> MPYTWKFLGISKQLSLENGIAKLNQLLNLEVDLDIQTIRVPSDPDGGTAADEYIRYEMRLDISNLDEGTYSKFIFLGNSKMEVPMFLCYCGTDNRNEVVLQWLKAEYGVIMWPIKFEQKTMIKLADASIVHVTKENIEQITWFSSKLYFEPETQDKNLRQFSIEIPRESCEGLALGYGNTMHPYNDAIVPYIYNETGMAVERLPLTSVILAGHTKIMRESIVTSTRSLRNRVLAVVLQSIQFTSE;> MSNELRLEDNYVPTSDTLVVFKQLMKLPVTVLYDLTLSWFAKFGGSFDGDIYLLTETLDLLIEKGVRRNVIVNRILYVYWPDGLNVFQLAEIDCHLMISKPEKFKWLPSKALRGDGKPYVVKLQPAKFIENLQTDLAKIYHCHVYMFKHPSLPVLITRIQLFDSNNLFLSTPNIGSINKESLYNKLDKFQGKPLISRRPYYVAFPLNSPIIFHSVDKDIYARLVLQSISRTISERETIIFKPVQKIPVKSIHNIMTLLGPSRFAESMGPWECYASANFERSPLHDYKKHQGLTGKKVMVREFDDSFLNDDENFYGKEEPEIRRLRLEKNMIKFKGSANGVMDQKYNDLKEFNEHVHNIRNGKKNEDSGEPVYISRYSSLVPIEKVGFTLKNEINSRIITIKLKFNGNDIFGGLHELCDKNLINIDKVPGWLAGENGSFSGTIMNGDFQREQVAKGGLLENLYFQ;> MSRIDDLQQDIESLLSEINSLEESREKLKAKIKDKRKNEESANPIVQEFEDLFDQFPQLNNFLFNEHPELEETDDKDISRAQADIPATPIPYEPKKRAKLENEEILPEQEWVLKTQPMVQHQMFDPGVADLLDTDILTSPSKRKRKLKIDDISTSDRSELEDYIVLENVYRMFGITFFPLVDPIDLKIKDASGEIFVDREMLGIRLEVFSERTSQFEKPHYVLLKKRIKSNSWFLFKHTIPSFIDVQGIFDDTNGGLVISHDDAYLFAKRVFLQLVEVQKRRQIFKDLEAKKIIHDLDLDLESSMVSFFVKDIKVELFVKQNEIVSCSILDDIHDFSQNNKSKWEIALLGSLDDLELKLNHSFATIFK;> MDFTSDTTNSHDTSNSHLSLEDAVGTHHAGEADVNIDGDEKQQLSLLDDDQVRALKLQEEKDALLTRRNTLLQEIQTYQNILMKENNSKTKNGDILQNDITQDFLNLISISSSNPNSAISDRKRVERINGLTNLQKELVTKYDTLPLLNMNLRLSYLRDHTYPHLQVSVQSRDRVHNDGIEVLVVNYKFCRNTMNPFEIQFKMFYKFEDSTLLKWEILRISTNVRLKAKQLLATRNFQKCLLSLYEFDKIKSKKTGIFQNLINLLKRKTRCYLMNNSDSLIVERVIREGRLTTIKLQINFIITMPGERGKPRNCFLPMSKISIALWKGGERF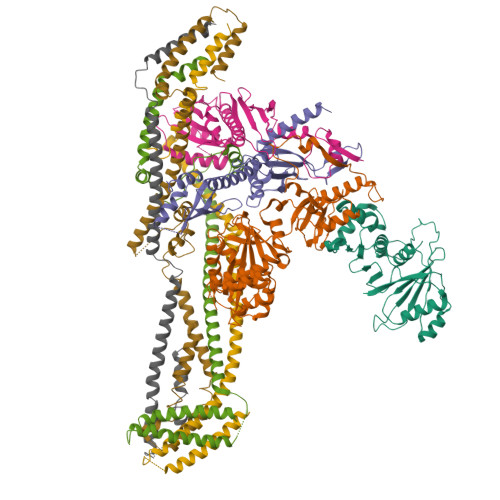NQIDLDEICYGLIKEYGVKTGLKEICNVCLFPDMYAR;> MAADRDNFLQNIENDSINNGQAMDLSPNRSSSESDSSILMNVNDIKTLRLDVAPEAKSTQSKKSLFYENSDDAEEGEIEERTNKEEGQYHHKGSKQLRFEVGKESTGKLQSHLSDGSATSGEGNVRPWEFRKVIQAEYRERLPRNYELKHWKKPSKIMIGSILRLLETNTVSALDSVFEKYEKEMNQMTHGDNNEVKRIYSKKERLLEIILTKIKKKLRQAKFPSRISERDLDIEYIYSKRQFIQNRYSQELQNNERLEAILSREQNLLEETRKLCMNLKTNNKKRLTEKLIQKDLHPVLNKAMEYTYGLESTNGFMHPDGPVTFRNDSHELNLMLNDPIKSTADVRLDKEEVLSLLPSLKEYTKKSKELKETMGQMISDSHEEEIKEVFVPHHESHQDKTEEDIH;> MDRDTKLAFRLRGSHSRRTDDIDDDVIVFKTPNAVYREENSPIQSPVQPILSSPKLANSFEFPITTNNVNAQDRHEHGYQPLDAEDYPMIDSENKSLISESPQNVRNDEDLTTRYNFDDIPIRQLSSSITSVTTIDVLSSLFINLFENDLIPQALKDFNKSDDDQFRKLLYKLDLRLFQTISDQMTRDLKDILDINVSNNELCYQLKQVLARKEDLNQQIISVRNEIQELKAGKDWHDLQNEQAKLNDKVKLNKRLNDLTSTLLGKYEGDRKIMSQDSEDDSIRDDSNILDIAHFVDLMDPYNGLLKKINKINENLSNEL;> MTDTYNSISNFIENELTALLSSDDYLMDDLAGELPNEVCRLLKAQVIEKRKDAMSRGKQDLLSKEIYDNESELRASQSQQIMELVGDIPKYSLGSELRNRVEGEPQSTSIERLIEDVLKLPQMEVADEEEVEVENDLKVLSEYSNLRKDLILKCQALQIGESKLSDILSQTNSINSLTTSIKEASEDDDISEYFATYNGKLVVALEEMKLLLEEAVKTFGNSPEKREKIKKILSELKK;> MNSEQLLHNYVSDSLLTTLISFQEFKQQLQSYTSDEQQLQHWYELLQARDARVTSELEARIKQFFITLRSRLLRFLESEQLSHSLSLETLIDALYKINDLLQQRLQILDDAIQEKTSELAEFENMVRSPSAGDNAIPGLLQIIQSYINLLEEN> PELPEVETVRRELEKRIVGQKIISIEATYPRMVLTGFEQLKKELTGKTIQGISRRGKYLIFEIGDDFRLISHLRMEGKYRLATLDAPREKHDHLTMKFADGQLIYADVRKFGTWELISTDQVLPYFLKKKIGPEPTYEDFDEKLFREKLRKSTKKIKPYLLEQTLVAGLGNIYVDEVLWLAKIHPEKETNQLIESSIHLLHDSIIEILQKAIKLGGSSIRTYSALGSTGKMQNELQVYGKTGEKCSGCGAEIQKIKVAGRGTHFCPVCQQK

The Fpg/Nei superfamily (also called H2TH superfamily) includes bi-functional enzymes able to remove a wide variety of oxidized bases. The enzyme architecture consists in two globular domains connected by a flexible hinge: (i) a N-terminal domain rich in β-structures containing a highly conserved N-terminal α-helix (αA) displaying generally a proline (P1) at the N-terminal involved in catalysis and (ii) a C-terminal domain rich in α-structures containing both DNA binding domains of the enzyme (the H2TH motif and a β-hairpin domain structured in most cases as a Zinc finger). All these enzymes feature AP lyase activity consisting in the successive cleavage at the 3’ and then at the 5’ sides of the abasic (AP) site according to β,δ-elimination. In this work, we deciphered at the atomic level the structural and/or functional determinants required for the specific inhibition of ZnF Fpg/Nei DNA glycosylases by the uncompetitive inhibitor 2TX.

Four LlFpg variants were constructed: W179A, R247G, C248GH and C268H. The aim of constructing these point mutations was to (i) disrupt the 2TX binding site (W179A), (ii) increase the C268 thiolate reactivity (R247G) or (iii)inactivate the reactive sites C248 or C268 by replacing C to H (C248GH, which mimics the situation found in hNEIL2, Supplementary Figure S1c; C268H). The crystal structures of R247G and C248GH bound to 14-mer THF-DNA have been solved and indicate that these point mutations do not affect the overall structure of ZnF as compared to the wild-type enzyme. Residues W179 and R247 are clearly involved in the second shell of the Zn-coordination sphere of LlFpg by establishing NH—S hydrogen bonds (from residue backbone and/or basic side chain with Cysteine thiolates). To evaluate the 2TX sensitivity of R247G and C248GH, we used the PAR assay. 2TX is able to extract the zinc ion from ZnF of R247G 3-times faster than it does with the wild-type enzyme. Assuming that the PAR assay is another manner to estimate the inhibition efficiency of the enzyme, the variant R247G appears more sensitive than the wild-type enzyme. As expected by 3D structures, the suppression of NH—S bonds from the second coordination shell of ZnF increases the reactivity of ZnF thiolates in the variant R247G and probably also the accessibility to W179 for binding.1-(2-{5-[(3-Methyloxetan-3-yl)methoxy]-1H-benzimidazol-1-yl}quinolin-8-yl)piperidin-4-amine | C26 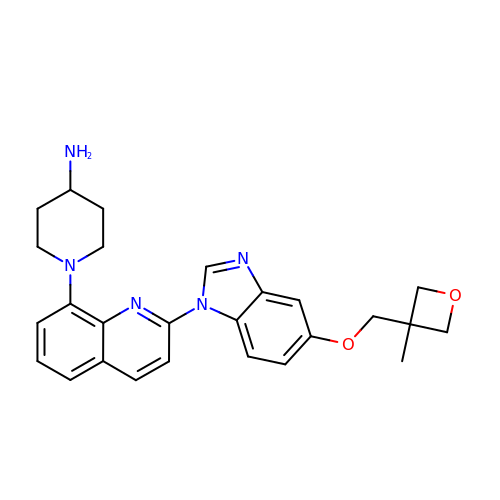H29 N5 O2 | DYNHJHQFHQTFTP-UHFFFAOYSA-N> MKGIIFTEFLDLVEDKFGLEMVDKIITQSELESEGVYTSIGTYRFSEMLQLLQNLSANTDVSIDDLLLTYGEHFFSVIEDSYPGLLATYKDPIEMLASIENHIHVEVRKIYPDAELPTFVVEEKTANSLT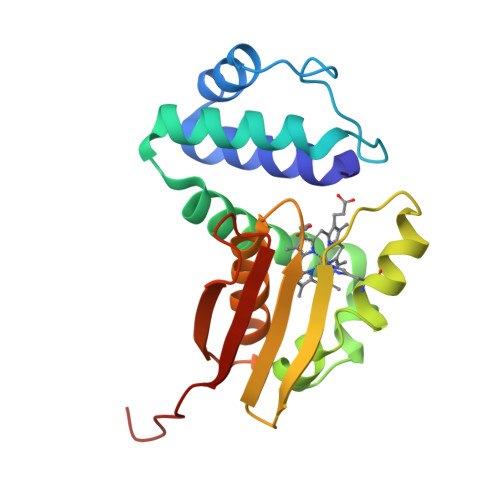MIYKSSRAMHHFGLGLMNKTFEHFNSSAEIILEKIKEDGTEVKFIINKNENLYFQ Several natural systems exhibit ‘facilitated dissociation’, in which an effector (E) can bind to a target–host (TH) complex to form an excited ternary complex (THE)20–26 from which the target dissociates quickly. We set out to design protein systems that undergo facilitated dissociation. We use a switchable target binder (host) and a flexible effector that can rapidly bind to and switch the target–host complex to induce a large steric clash with the target, forming a strained excited ternary complex. We show here that by explicitly considering excited intermediate states when designing coupled protein systems, a broad range of facilitated dissociation systems can be designed.

We used X-ray crystallography to structurally characterize multiple states of our designed systems. For both the AS1 and the AS5 systems, the crystal structures of the hosts alone and of the host–effector complexes closely match the design models (maximum 1.3 Å Cα root mean square deviation (RMSD)). The unbound structures show an open hydrophobic cleft in the new designed state X poised to bind the effector, and the effector-bound structures show that binding the effector causes the two switch domains to register-shift into the designed state Y. Crystal structures throughout the facilitated dissociation process confirm our ability to design excited states and large register-shift conformational changes.

> MSGSLREEIRKLAEQLSEKYKDEEIRELAREAAELAEESDDPEVLELAYEALKKGLELEDEEKVKLILLAAVLAARVARGEVPEEKLEIALKALELAEASEDERIIRGALRAALAAARTDDPLALEVVLEALERAQASEDERLIRAILAAAYAFALLAVAGASAERLKEAEAIVKELIAAAEKGASPQELVLLVIEMMVKGMGVTMETHRSGNEVKVVIKGLHESQQEVLLEAVLFAAELMGVRVRIRFKGDTVTIVVRE;> EERKKELAKEVIETAKKLIEKLAKEE> MTSIKPFQMEDLFELNPVNLDPLTENFNVSFYSQYLIEWPQLFYKSVETPNGQASGYMMAKTEGQLSKKEWHTHITAVTVLDQYRRIGLASKL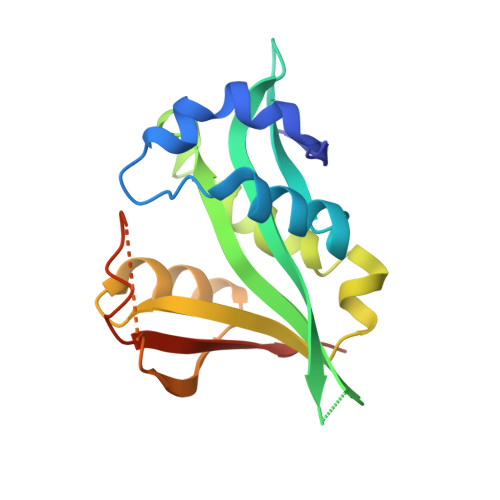CLELENLTQVKDTLFIDLFVKVTNTLGRILYEKLGYSVFRRVVGYYGREIQKDRNKIDDSVDAFDMRKLLPRDVNNE>SCSFDGRIAFYRFCNLTQVPQVLNTTERLLLSFNYIRTVTASSFPFLEQLQLLELGSQYTPLTIDKEAFRNLPNLRILDLGSSKIYFLHPDAFQGLFHLFELRLYFCGLSDAVLKDGYFRNLKALTRLDLSKNQIRSLYLHPSFGKLNSLKSIDFSSNQIFLVCEHELEPLQGKTLSFFSLAANSLYSRVSVDWGKCMNPFRNMVLEILDVSGNGWTVDITGNFSNAISKSQAFSLILAHHIMGAGFGFHNIKDPDQNTFAGLARSSVRHLDLSHGFVFSLNSRVFETLKDLKVLNLAYNKINKIADEAFYGLDNLQVLNLSYNLLGELYSSNFYGLPKVAYIDLQKNHIAIIQDQTFKFLEKLQTLDLRDNALTTIHFIPSIPDIFLSGNKLVTLPKINLTANLIHLSENRLENLDILYFLLRVPHLQILILNQNRFSSCSGDQTPSENPSLEQLFLGENMLQLAWETELCWDVFEGLSHLQVLYLNHNYLNSLPPGVFSHLTALRGLSLNSNRLTVLSHNDLPANLEILDISRNQLLAPNPDVFVSLSVLDITHNKFICECELSTFINWLNHTNVTIAGPPADIYCVYPDSFSGVSLFSLSTEGCDEEEVLKSLKFSLFIVCTVTLTLFLMTILTVTKFRGFCFICYKTAQRLVFKDHPQGTEPDMYKYDAYLCFSSKDFTWVQNALLKHLDTQYSDQNRFNLCF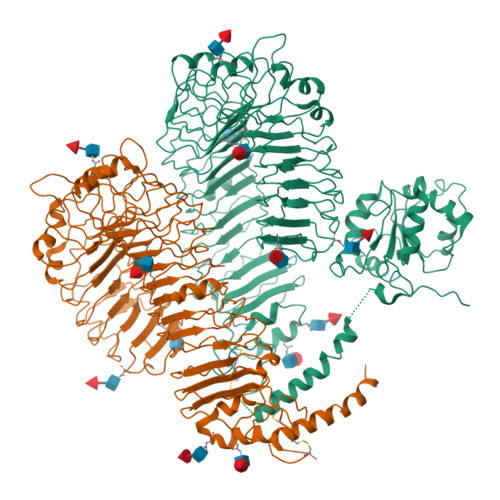EERDFVPGENRIANIQDAIWNSRKIVCLVSRHFLRDGWCLEAFSYAQGRCLSDLNSALIMVVVGSLSQYQLMKHQSIRGFVQKQQYLRWPEDFQDVGWFLHKLSQQILKKEKEKKKDNNIPLQTVATISGSHHHHHH[2x]> MGSSHHHHHHGTGSYITSLYKKAGWGSNEAQVKKESIGEIMGKLMQGEIGDEELSKRIKEIFGKRLQWGYKPTHQQQLAFNLDFIKSLKEMDMSGEIDTMNEETYELPSAFLEAAFGKTIKQSGCYFKDETTTIDEAEEASHELYCERAQIKDGQTVLDIGCGQGGLVLHIAQKYKNCHVTGLTNSKAQKNYILMQAEKLQLSNVDVILADVTKHESDKTYDRILVIATIEHMKNIQLFMKKLSTWMTEDSLLFVDHICHKTFSHHFEAIDEDDWYSGFIFPKGCVTILSASALLYFQDDVTILDHWVVNGMHMARSVDAWRKKLDKNMELAREILLPGLGSKEAVNGVITHIRTFCMGGYEQFSYNNGEEWMVAQMLFK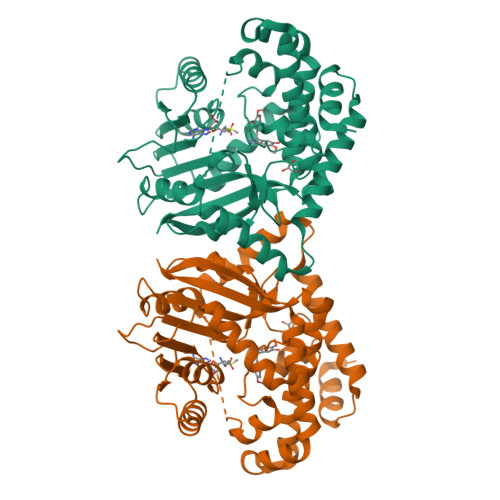KK>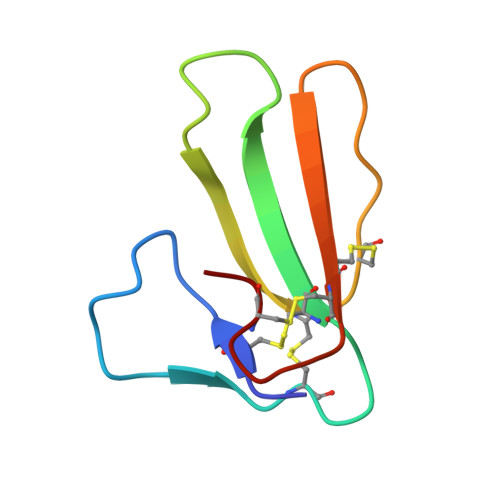 TMCYSHTTTSRAILTNCGENSCYRKSRRHPPKMVLGRGCGCPPGDDYLEVKCCTSPDKCNY> SMSSFEGQMAEYPTISIDRFDRENLRARAYFLSHCHKAHMKGLRAPTLKRRLECSLKV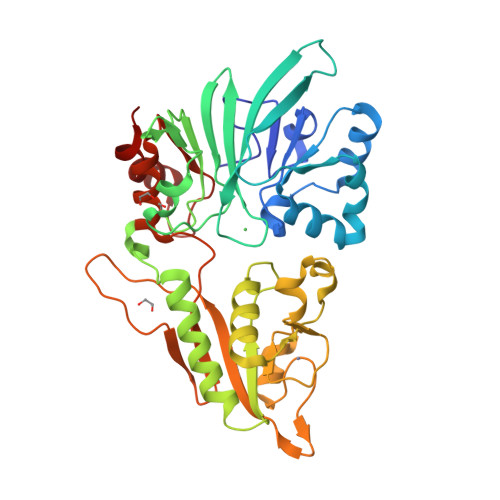YLYCSPVTKELLLTSPKYRFWKKRIISIEIETPTQISLVDEASGEKEEIVVTLLPAGHCPGSVMFLFQGNNGTVLYTGDFRLAQGEAARMELLHSGGRVKDIQSVYLDTTFCDPRFYQIPSREECLSGVLELVRSWITRSPYHVVWLNCKAAYGYEYLFTNLSEELGVQVHVNKLDMFRNMPEILHHLTTDRNTQIHACRHPKAEEYFQWSKLPCGITSRNRIPLHIISIKPSTMWFGERSRKTNVIVRTGESSYRACFSFHSSYSEIKDFLSYLCPVNAYPNVIPVGTTMDKVVEILKPLCRS9-HYDROXY ARISTOLOCHIC ACID | C17 H11 N O8 | 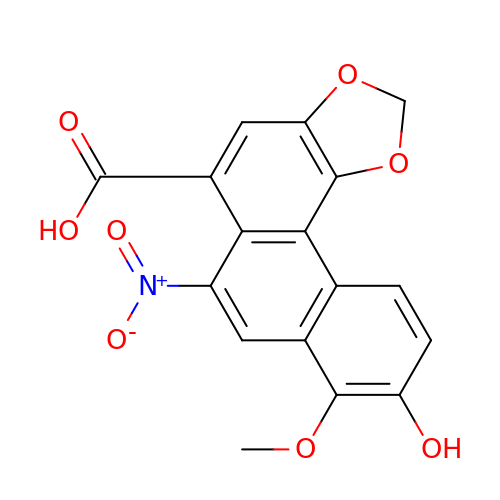UCLGCTLOEZZSLA-UHFFFAOYSA-N>GPMKRGFARPTPEKPPVIGSSGQESADSMDANYRWFHPAPNTLAAAVGSPRMWERKPDGKDLNFGVVRVGGSGFGRYQSVVYNLPKMVSLLVEPWYALVGEREQVLGLMRAIICQLAFSHGPDHVQMIVVSSDLDQWDWVKWLPHFGDSRRHDAAGNARMVYTSVREFAAEQAELFAGRGSFTPRHASSSAQTPTPHTVIIADVDDPQ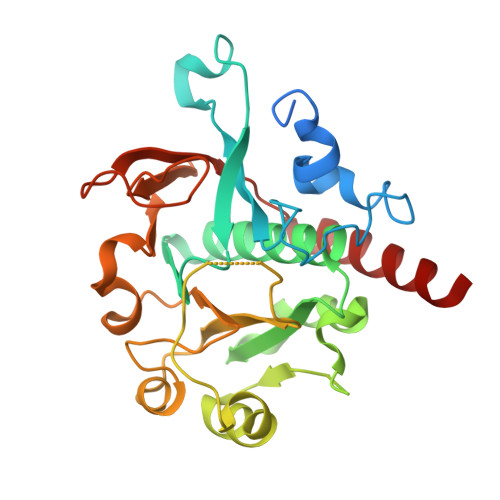WEYVISAEGVDGVTFFDLTGSSMWTDIPERKLQFDKTGVIEALPRDRDTWMVIDDKAWFFALTDQVSIAEAEEFAQKLAQWRLA[2x]> MERAPLLELKGIRKRFGELEVLRGVDLALYPGEILALLGPSGCGKTTLLRVVAGLEVPDAGRVFLEGRDITALPPEKRGIGFVFQDYALFPHLTALGNVAFGLKGKDRLARARKALERVG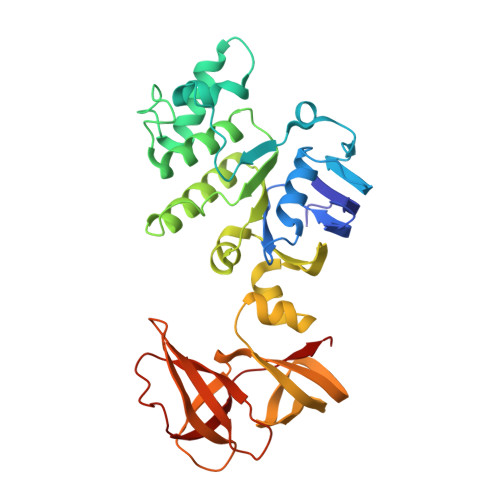MTLFQDRRPGELSGGQQQRVALARALAPGPKLVLLDEPFSSLDAGLRAATREEVRKVLKETGTAALLVTHDQEEALSFADRLGVMRGGEILQVGTPEEVYLRPKTPFVAQFLGRTNLLPGEGRGRYAETCLGRVPLAEAREGPLLLSLRPEALRLTPPGQGPQGEVVAREFKGHDLTYRVRLHGVQPEREVLVQEGPTCPFKVGDRVGLEVVGEGVALEG>[12x]EKFLVIAGPNAIESEELLLKVGEEIKRLSEKFKEVEFVFKSSFDKANRSSIHSFRGHGLEYGVKALRKVKEEFGLKITTDIHESWQAEPVAEVADIIQIPAFLCRQTDLLLAAAKTGRAVNVKKGQFLAPWDTKNVVEK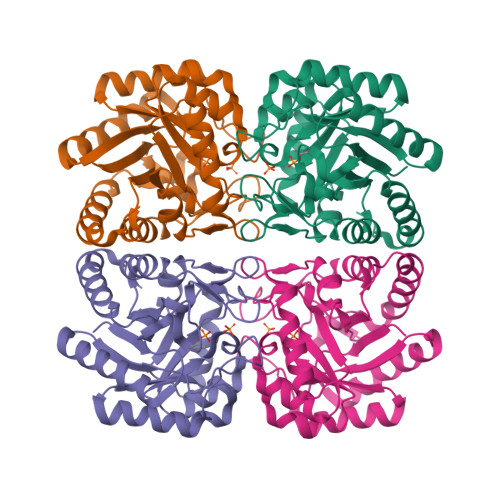LKFGGAKEIYLTERGTTFGYNNLVVDFRSLPIMKQWAKVIYDATHSVQLPGGLGDKSGGMREFIFPLIRAAVAVGCDGVFMETHPEPEKALSDAPTALPLSQLEGIIEAILEIREVASKYYETI Our research group has been studying a representative FAD-dependent dehydrogenase complex (FADGDH) derived from Burkholderia cepacia SM4 (BcGDH). Owing to the presence of the β-subunit, BcGDH is capable of transferring electrons directly to an electrode, making it an ideal molecule for glucose sensors and applications in a variety of biomedical devices. In this study, we determined the X-ray structure of BcGDHγα, consisting of the BcGDH catalytic subunit complexed with the small (hitchhiker) subunit. The structure of BcGDHγα revealed a conserved GMC oxidoreductase-type scaffold and a His/Asn catalytic pair, with a unique structure of the 3Fe–4S cluster, which serves as the electron acceptor of FAD and simultaneously serves as the electron donor for electron transfer of the multiheme c subunit.

In the crystal, two pairs of BcGDHγα complexes were observed in the asymmetric unit. Therefore, the observed γαγ′α′ heterotetramer in the crystal structure is an artifact of crystallization. FAD is surrounded by part of the long loop between Ala98 and Ser109, α1, α15, β2 and β6. Since continuous electron density was observed between FAD and His105 in the α-subunit of BcGDHγα [Fig. 2(b)], a covalent bond was deemed to form between FAD and His105 in the α-subunit of BcGDH. The simulated-annealing OMIT maps of sulfur ions in the iron–sulfur cluster and the disulfide bond indicated that this iron–sulfur cluster is a 3Fe–4S cluster coordinated by Cys212, Cys218 and Cys222 of the α-subunit. A neighboring cysteine, Cys213, in the α-subunit forms a disulfide bond with Cys152 of the γ-subunit. The unique cysteine cluster of BcGDHγα contributes to the formation of the 3Fe–4S cluster for electron transfer and the disulfide bond for stabilization of the structure of the γα complex. The γ-subunit tightly binds the α-subunit and forms a stable heterodimer. The distance between N5 of FAD and the 3Fe–4S cluster is about 12–13 Å, which is an adequate distance for electron transfer. The catalytic pair in BcGDH is likely to be His/Asn, represented by His476 and Asn519, and corresponds to His689 and Asn732 in cellobiose dehydro­genase.

>DNPGTAPLDTFMTLSESLTGKKGLSRVIGERLLQALQKGSFKTADSLPQLAGALASGSLTPEQESLALTILEAWYLGIVDNVVITYEEALMFGVVSDTLVIRSYCPNKPGFWADKPIERQA[2x];>[2x]MADTDTQKADVVVVGSGVAGAIVAHQLAMAGKAVILLEAGPRMPRWEIVERFRNQPDKMDFMAPYPSSPWAPHPEYGPPNDYLILKGEHKFNSQYIRAVGGTTWHWAASAWRFIPNDFKMKSVYGVGRDWPIQYDDLEPYYQRAEEELGVWGPGPEEDLYSPRKQPYPMPPLPLSFNEQTIKTALNNYDPKFHVVTEPVARNSRPYDGRPTCCGNNNCMPICPIGAMYNGIVHVEKAERAGAKLIENAVVYKLETGPDKRIVAALYKDKTGAEHRVEGKYFVLAANGIETPKILLMSANRDFPNGVANSSDMVGRNLMDHPGTGVSFYASEKLWPGRGPQEMTSLIGFRDGPFRATEAAKKIHLSNLSRIDQETQKIFKAGKLMKPDELDAQIRDRSARYVQFDCFHEILPQPENRIVPSKTATDAIGIPRPEITYAIDDYVKRGAAHTREVYATAAKVLGGTDVVFNDEFAPNNHITGSTIMGADARDSVVDKDCRTFDHPNLFISSSATMPTVGTVNVTLTIAALALRMSDTLKKEVHHHHHH> A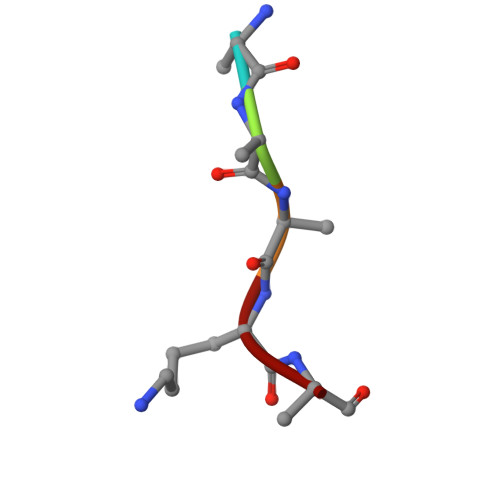AAKA>[2x]MLIIGERINGMFGDIKRAIQERDPAPVQEWARRQEEGGARALDLNVGPAVQDKVSAMEWLVEVTQEVSNLTLCLDSTNIK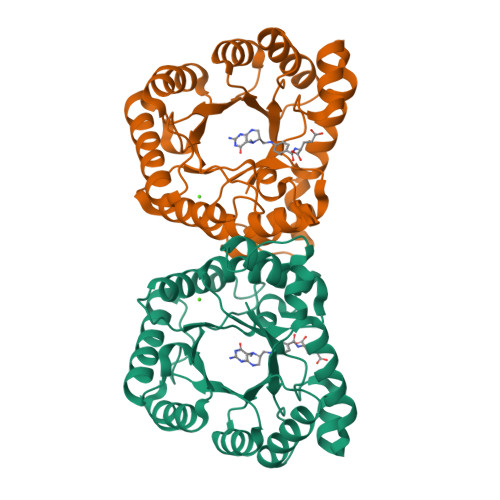AIEAGLKKCKNRAMINSTNAEREKVEKLFPLAVEHGAALIGLTMNKTGIPKDSDTRLAFAMELVAAADEFGLPMEDLYIDPLILPANVAQDHAPEVLKTLQQIKMLADPAPKTVLGLSAVSQNCQNRPLINRTFLAMAMACGLDAAIADACDEALIETAATAEILLNQTVYCDSFVKMFKTR> FACKTANGTAIPIGGGSANVYVNLAPVVNVGQNLVVDLSTQIFCHNDYPETITDYVTLQRGAAYGGVLSSFSGTVKYNGSSYPFPTTSETPRVVYNSRTDKPWPVALYLTPVSSAGGVAIKAGSLIAVLILRQTNNYNSDDFQFVWNIYANNDV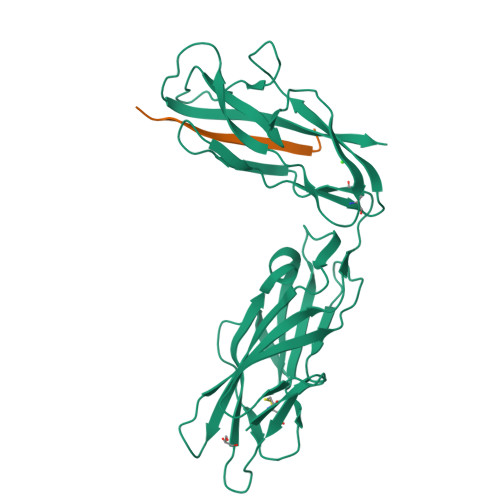VVPTGGCDASARDVTVTLPDYPGSVPIPLTVYCAKSQNLGYYLSGTTADAGNSIFTNTASFSPAQGVGVQLTRNGTIIPANNTVSLGAVGTSAVSLGLTANYARTGGQVTAGNVQSIIGVTFVYQ;> ADVTITVNGKVVAKP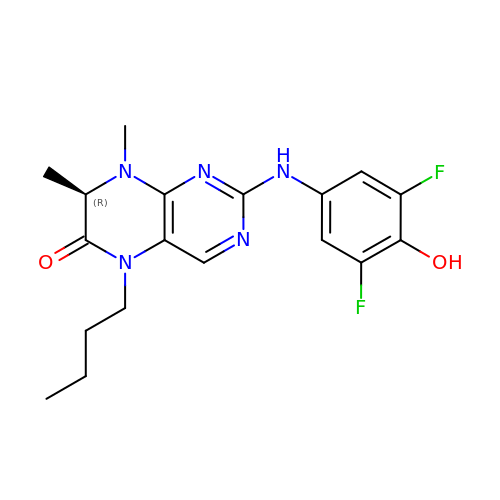(7R)-5-butyl-2-[(3,5-difluoro-4-hydroxyphenyl)amino]-7,8-dimethyl-7,8-dihydropteridin-6(5H)-one | C18 H21 F2 N5 O2 | IQHUYDHFNRXPGH-SNVBAGLBSA-N> GPLGSTAFRKFYERGDFPIALEHDSKGNKIAWKVEIEKLDYHHYLPLFFDGLCEMTFPYEFFARQGIHDMLEHGGNKILPVLPQLIIPIKNALNLRNRQVICVTLKVLQHLVVSAEMVGKALVPYYRQILPVLNIFKNMNVNSGDGID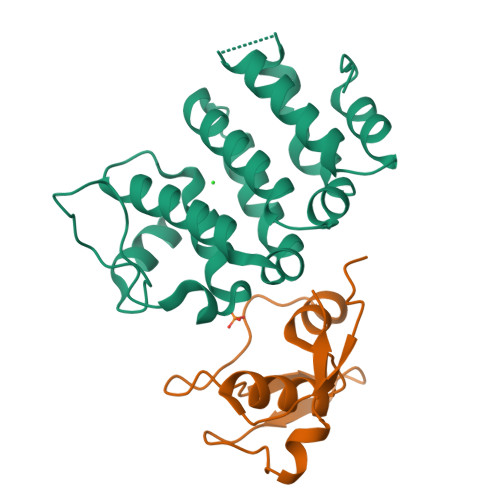YSQQKRENIGDLIQETLEAFERYGGENAFINIKYVVPTYESCLLN;> GPLGSMASSDVKPKSVSHAKKWSEEIENLYRFQQAGYRDETEYRQVKQVSMVDRWPETGYVKKLQRRDNTFYYYNKQRECDDKEVHKVKIYAY> SLSNKLTLDKLDVKGKRVVMRVDFNVPMKNNQITNNQRIKAAVPSIKFCLDNGAKSVVLMSHLGRPDGVPMPDKYSLEPVAVELKSLLGKDVLFLKDCVGPEVEKACANPAAGSVILLENLRFHVEEEGKGKDASGNKVKAEPAKIEAFRASLSKLGDVYVNDAFGTAHRAHSSMVGVNLPQKAGGFLIKKELNYFAKALESPERPFLAILGGAKVADKIQLINNMLDKVNEMIIGGGMAFTFLKVLNNMEIGTSLFDEEGAKIVKDLMSKAEKNGVKITLPVDFVTADKFDENAKTGQATVASGIPAGWMGLDCGPESSKKYAEAVTRAKQIVWNGPVGVFEWEAFARGTKALMDEVVKATSRGCITIIGGGDTATCCAKWNTEDKVSHVSTGGGASLELLEGKVLPGVDALSNI

Phosphoglycerate kinase 1 (PGK1) is an ubiquitous enzyme expressed in all somatic cells that plays a central role in glycolysis where it provides energy in form of ATP through the reversible phosphotransfer reaction from 1,3-bisphosphoglycerate (1,3-BPG) to MgADP in order to produce 3-phosphoglycerate (3-PG) and MgATP in the presence of free magnesium. PGK1 is a monomeric enzyme of 417 amino acids formed by two distinct α-helical domains of equal size, the N- and C-terminal domains connected by a hinge region. The N-terminal domain binds 3-PG or 1,3-BPG while the C-terminal domain binds MgADP or MgATP. Two different crystallographic conformations of PGK1 have been already identified: the partially closed conformation, able to bind substrates, and the closed conformation, the catalytically competent state.

Residue 189 is part of the 189–201 α-helix, the structural element that represents the hinge connecting the N-terminal 3-PG binding domain and the C-terminal ADP binding domain. Another form, defined as open and that is the most populated conformation in solution, has been detected through small-angle X-ray scattering. It is interesting to note that all the mutants crystallized in the partially closed conformation but only M189I crystallized even in the closed form, suggesting that for the variants R38M, G166D and V216F the closed form is less favourable in the crystallization conditions. We solved the structures of all these mutants in the partially closed conformation, and we succeed to solve the structure of M189I also in the totally closed conformation. The structure appear to be identical to the wild type ones; also the position of the two ligands, ADP and 3-PG, is conserved. Interestingly, in the M189I structure in the closed conformation MgF3- is not present, therefore the transition complex, evident in the wild type structure, is not formed in the M189I variant. Nevertheless, all the residues stabilizing the transition state are superposable between the wild type and mutant structure.>[4x]MSGDGS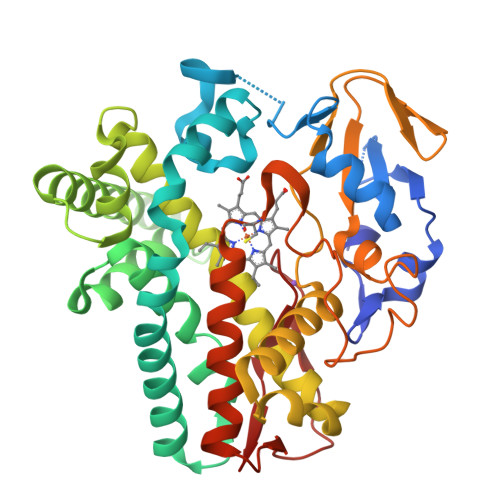PPIHTRRQGFDPADELRAAGTLTKISIGSGADAETTWLAAGHAVVRQVLGDHQQFSTRRRWDPRDEIGGKGIFRPRELVGNLMDYDPPEHTRLRHLLTPGFTQRRMRRLAPRIEEIVTDRLDAMEQAGPPADLIELFADEVPGAVLCELIGVPRDDRDMFMKLCHGHLDASLSQKRRAALGDKFSRYLLAMIARERKDPGDGFIGSIVAEHGDTITDEELRGVCVQLMLAGDDNVSGMIGLGVLALLRHPEQIAALRGDDQSADRAVDELIRYLTVPYAPTPRTAVEDVMVADQVIKEGETVLCSLPMANRDRALLPDADRLDVTRTPVPHVAFGHGIHHCLGAALTRLQLRIAYTALWRRFPALQLADPAQEIMFRTSTPAYGLTSLLVAW>SQALKNLLTLLNLEKIEEGLFRGQSEDLGLRQVFGGQVVGQALYAAKETVPEERLVHSFHSYFLRPGDSKKPIIYDVETLRDGNSFSARRVAAIQNGKPIFYMTASFQAPEAGFEHQKTMPSAPA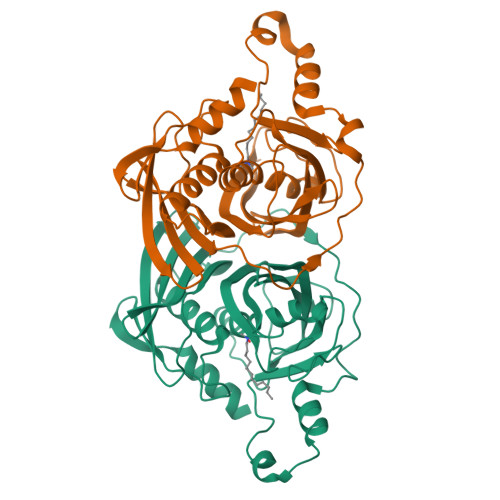PDGLPSETQIAQSLAHLLPPVLKDKFICDRPLEVRPVEFHNPLKGHVAEPHRQVWIRANGSVPDDLRVHQYLLGYASDLNFLPVALQPHGIGFLEPGIQIATIDHSMWFHRPFNLNEWLLYSVESTSASSARGFVRGEFYTQDGVLVASTVQEGVMRNHN[2x]PGAM5 is a mitochondrial membrane protein that functions as an atypical Ser/Thr phosphatase and is a regulator of oxidative stress response, necroptosis, and autophagy. Phosphoglycerate mutase family member 5 (PGAM5) is a mitochondrial membrane protein that belongs to the phosphoglycerate mutase (PGAM) branch of the histidine acid phosphatase superfamily, known also as two-histidine phosphatase (2H-phosphatase). Despite harboring a canonical RHGE catalytic motif, PGAM5 lacks a typical phosphotransferase and/or phosphohydrolase activity for small metabolites, and displays instead a phosphatase function specific for Ser/Thr and, potentially, histidine residues (Takeda et al., 2009, Panda et al., 2016). Overall, the catalytic domain of PGAM5 adopted a classical phosphoglycerate mutase-like fold with the canonical three-layer sandwich topology, which featured a six-stranded β sheet flanked on both sides by α helices with the first four parallel strands arranged in an alternated β/α manner.

To provide high-resolution details of the catalytic center, we also determined the high-resolution structure of ΔN90-PGAM5 in complex with phosphate. The β3-α3 loop was the region that showed the highest degree of flexibility with two major conformations observed, an opened form in the apo and off states and a closed form in the on state (root-mean-square deviation [RMSD] of ∼0.9 Å with an average Cα shift of ∼3.9 Å for residues 175–179). Binding of a phosphate ion induced a number of rearrangements in the active site resulting in two distinct on and off states, which were termed in relation to the “in” and “out” conformation of H105, respectively. In the on state, in addition to H105 all catalytic residues were observed to assume a potentially catalytically active position. This conformation was most likely induced by the closure of the β3-α3 loop which moved E177 inward, triggering an inward swing of H230. In a concerted manner, the “in” H230 likely forced an approximately 90° rotation of R152 side chain orienting perpendicular to H105 and planar to Y108 for cation-π stacking. In comparison, the stark difference of the off state of the enzyme was characterized by an “out” position of H105, rotating away from its catalytically competent position. This movement was likely a consequence of steric constraints created by R104 and R152 that retained their “vertical” conformations. Although this conformation maintained affinity for phosphate, the all-out rearrangement of the catalytic residues presumably depicted a catalytically incompetent state of the enzyme.

>SMDHYKAKATRHIFLIRHSQYHVDGSLEKDRTLTPLGREQAELTGLRLASLGLKFNKIVHSSMTRAIETTDIISRHLPGVCKVSTDLLREGAPIEPDPPVSHWKPEAVQYYEDGARIEAAFRNYIHRADARQEEDSYEIFICHANVIRYIVCRALQFPPEGWLRLSLNNGSITHLVIRPNGRVALRTLGDTGFMPPDKITRS[2x]>KHSLPDLPYDYGALEPHINAQIMQLHHSKHHAAYVNNLNVTEEKYQEALAKGDVTAQIALQPALKFNGGGHINHSIFWTNLSPNGGGEPKGELLEAIKRDFGSFDKFKEKLTAASVGVQGSGWGWLGFNKERGHLQIAACPNQDPLQGTTGLIPLLGIDVWDHAYYLQYKNVRPD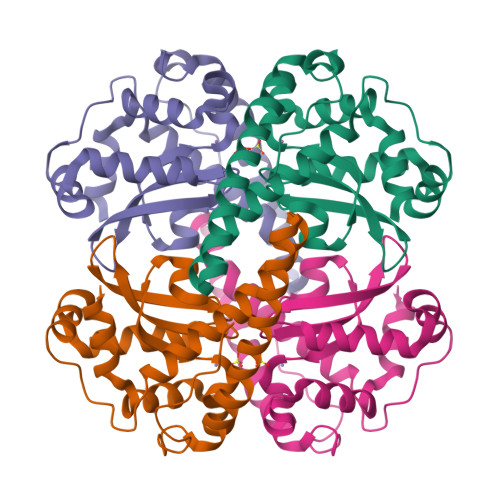YLKAIWNVINWENVTERYMACKK[2x]(3aS,4S,6aR)-2-oxo-hexahydro-1H-thieno[3,4- d]imidazolidin-4-yl]-N-{2-[(2,6- diphenylphenyl)formamido]ethyl}pentanamide | C31 H34 N4 O3 S | 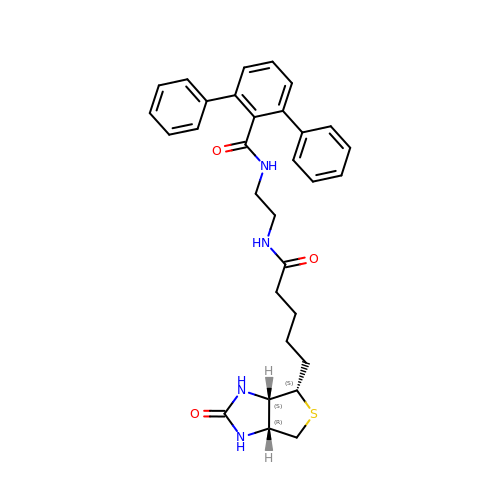HDCOHCMVDIFBPR-ZEZDXWPOSA-N> TKLIAQTFGNVALGGGGFVSGIISHKTSGDVYCRTDVGGAYRWDAVNSKWIPLLDWTSENETTYQGVEALALDPQNANNLYLLAGTAYFNGGKTAILKSTDKGNTFTEVIVTSQFTAHGNRLGRANGERLAVDPNNSSILFCGTGANGLWKSTNGGLTWTLAWNGVTTTSNGNGICFVVFDPSSVSGGVTQTIYIGVSRTGANNIYKSTDGGSTFTAIQPDNSFMPHRAVLSSDNSTLYVAMADGEGPSNGGSGRVYKLVTATGTWTNITPNGNNFPYGGVSVDPSNTNRIIVSTENAWSNNQFGATWGDFVFFSANGGNTWTQKLSSTSTLNTNGIGWIAGRGIHWAGSIDFDPLNTARVRVISGNGIFTCDDINASATSWKFDVKGMEETVVLDAISIPGGSFISAVGDQFGAVYSNVYAYPAKVHTPTVTSNNGIAYAANNVSKVVRATDQLYYSTDQGATWTAAASTIGGGYGKIALSADGNTTLYCPSGQSTTYYSTDNGGSWTSTGVTTVQDACPIADYVNTNKFYIYSPTSGQLLVST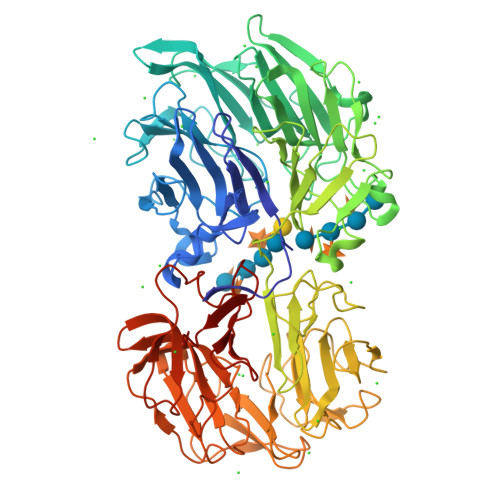NKGVSFTASAVNPGQWGSGRARAVPDNEGSVWVALNGGGLKYTTNNGTSWTTVPNVSYCGAVGIGKAATGATYPAVYIWGTVSGVRGMFRSTDQGASWIRINDDAHEWGGPGNGNFVMGDMNVFGRVYMSTVGRGLVTIESDLSALPLQFTH> TTILKHLPVGQRIGIAFSGGLDTSAALLWMRQKGAVPYAYTANLGQPDEEDYDAIPRRAMEYGAENARLIDCRKQLVAEGIAAIQCGAFHNTTGGLTYFNTTPLGRAVTGTMLVAAMKEDGVNIWGDGSTYKGNDIERFYRYGLLTNAELQIYKPWLDTDFIDELGGRHEMSEFMIACGFDYKMSVEKAYSTDSNMLGATHEAKDLEYLNSSVKIVNPIMGVKFWDESVKIPAEEVTVRFEQGHPVALNGKTFSDDVEMMLEANRIGGRHGLGMSDQIENRIIEAKSRGIYEAPGMALLHIAYERLLTGIHNEDTIE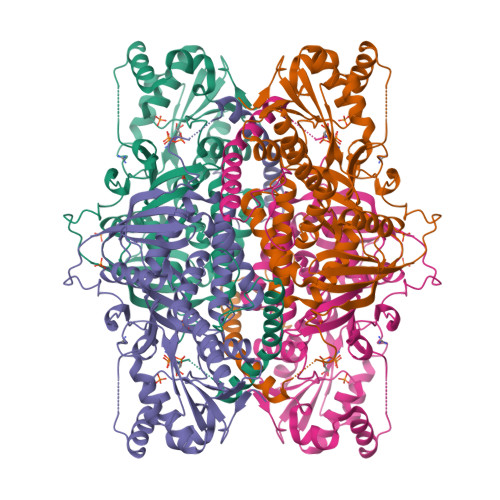QYHAHGRQLGRLLYQGRWFDSQALMLRDSLQRWVASQITGEVTLELRRGNDYSILNTVSENLTYKPERLTMEKGDSVFSPDDRIGQLTMRNLDITDTREKLFGYAKTGLLSSSAASGVPQVENLENKGQSVEHHHHHH> GGCUUCAUAUAAUCCGAAUGAUAUGGUUUCGGAGCUUCCAC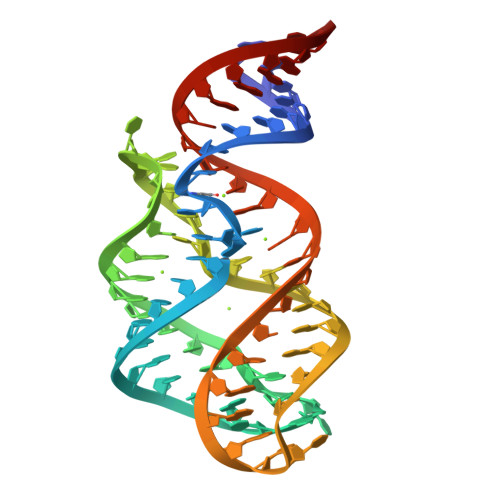CAAGAGCCUUAAACUCUUGACUAUGAAGUC> MKKNIIITLLAAASLTSCGEYNKLLKSTDYEYKYEAAKNYFAKGQYNRSATLLNELITILKGTDKAEESLYMLGMSYYNQKDY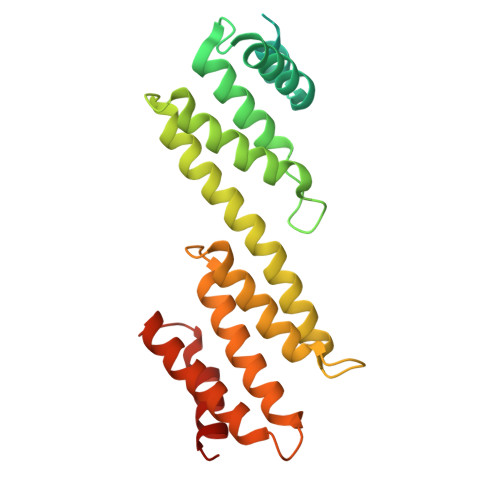QTAAQTFITYFNTYPRGTFTELARFHAGKSLFLDTPEPRLDQSSTYQAIQQLQMFMEYFPNSTKKQEAQDMIFALQDKLVLKELYSAKLYYNLGNYLGNNYESCVITAQNALKDYPYTDYREELSILILRARHEMAIYSVEDKKMDRYRETIDEYYAFKNEFPESKYLKEAEKIFNESQKVIKD Like E1 enzymes, aminoacyl tRNA synthetases (aaRSs) are adenylate-forming enzymes (AFEs). They catalyze the transformation of amino acids into AMP conjugates, and then into aminoacyl-tRNAs, to supply protein synthesis. PfYRS is a Class I aaRS, characterized by a catalytic domain that adopts a Rossmann fold (residues 18–260) linked to a C-terminal domain (residues 261–370) that is involved in recognition of the anticodon stem of tRNATyr. PfYRS contains the two motifs characteristic of the catalytic domain of Class I (sub-class c) tRNA synthetases: “HIGH” and “KMSKS” (70HIAQ73 and 247KMSKS251 in PfYRS).

Whereas formation of the AMP adenylate requires only Tyr and ATP, the thermal stabilization induced by ML901 required all three substrates (Tyr, ATP and tRNATyr).

>[2x]GMETTDTKREEQEIEEKKAQEESKIEDVDKILNDILSISSECIQPDELRVKLLLKRKLICYDGFEPSGRMHIAQGLLKSIIVNKLTSNGCTFIFWIADWFAHLNNKMSGDLKKIKKVGSYFIEVWKSCGMNMENVQFLWASEEINKKPNEYWSLVLDISRSFNINRMKRCLKIMGRSEGEENYCSQILYPCMQCADIFFLNVDICQLGIDQRKVNMLAREYCDIKKIKKKPVILSHGMLPGLLEGQEKMSKSDENSAIFMDDSESDVNRKIKKAYCPPNVIENNPIYAYAKSIIFPSYNEFNLVRKEKNGGDKTYYTLQELEHDYVNGFIHPLDLKDNVAMYINKLLQPVRDHFQNNIEAKNLLNEIKKYKVTK>[4x]MRGSHHHHHHGSMSYYNLEKDDTVYYKLDTIKCDIPINEELQARINKHVNQLRITYSTLEEFVDNFVYELKKGLEAHRRHPNLWIPHECSFKMLDSCIADIPTGQEKGTYYAIDFGGTNFRAVRASLDGNGKIKRDQETYSLKFTGTFSHEKGLLDKHATASQLFDHFAERIKYIMGEFKDLDNPEGKNVGFTFSFPCTSPSINCSILIDWTKGF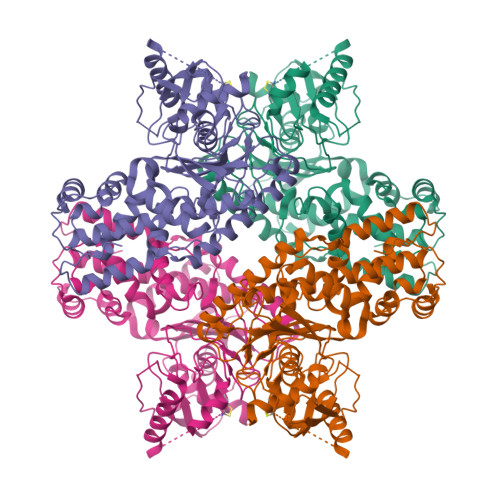ETGRATNDPVEGRDVCKLMNDAFVRSEVPAKVCCVVNDAVGTLMSCAYQKGKTTPPCYIGIILGTGSNGCYYEPEWKKYKYSGKIINIELGNFDKDLPLSPIDLVMDWHSANRSRQLFEKMISGAYLGEIVRRFMVNVLQSASSEKMWKSDSFNSELGSVVLNDTSPNFEESRKVAKDAWDMDFTDEQIYALRKICESVYNRSAALAAAAIAAIAKRIKIIEHSKFSCGVDGSLFVKNAWYCKRLQEHLKVILADKAENLIIIPADDGSGKGAAITAAVVSQSSSIKQLP2-phenyl-N-{5-[4-({5-[(phenylacetyl)amino]-1,3,4-thiadiazol-2-yl}amino)piperidin-1-yl]-1,3,4-thiadiazol-2-yl}acetamide 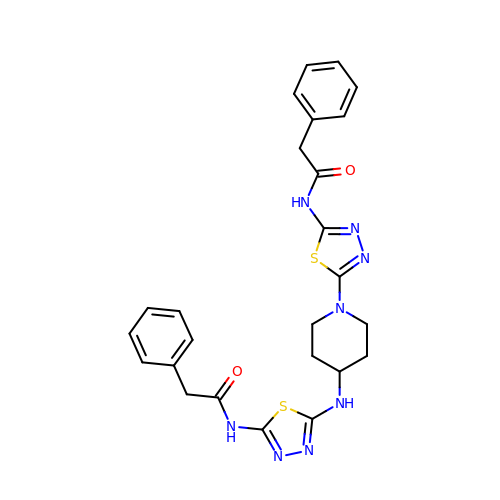| C25 H26 N8 O2 S2 | MRYCNTHLPRENBA-UHFFFAOYSA-N> MKLAQGAFVDVIRIGALSPPTDQRSLWARTLLSEAVDQGLDSLPVPLQDVSTFTVTLQPALAVRLKALADQHNTPVSVYAAGLIEAMRRRSESGSVAEAPMELPADALPGEGAVREVLRPLLKQAAEKTAAGKIVFAEAATGTGKGRMIASLAAAAAIKGDTVVVSAPLAVTWQLVNDMKDIPEVRRVGLTLSLGRPNFISPQRTLEWAIDNERADLAAWIEGGGKPLSLRSMETSKVISHELCWLLEDALLLAEDLPADSLLLTSEDPADCPAQQLYVAMRSNYTEAGIILCSHFMLAAHTRMMQMRGLGNDEELDDEAPTGLSLPHFIDTLIVDEAHLLEQAFASVYTHT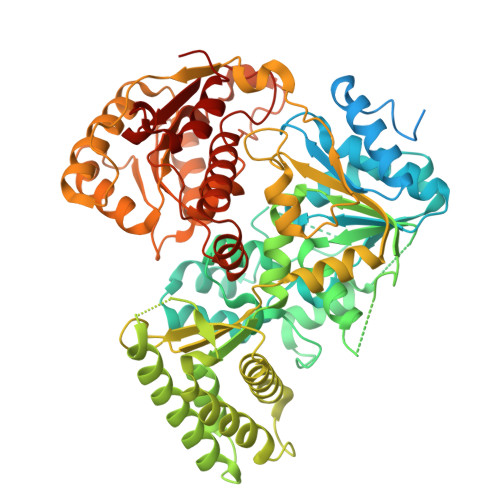LRLRPLMRTIEGLGSRGRKPALDALKELFTQMQVASARSTNTSLNVPLSDVPELIPALKDTVKTLGALPTKGMSRDARSVIRIATRAANDALSGHSRLRIEVTPVHSYPMLLSGRSNLQRALLGLWNATGGATLVSATLFTTGDNGSLTRWKLEVPTERAAFLPPVHPAWTTAPVLLHKEFCAHEPDDSPEWATECAQTIQGVASTAQGGTLVLCTSYQNTELLAGRLGAALGDRLIVQSKTSSAATCLAQFKAKHKAGIRPVWLGLGAAWTGIDLSDHSLPDNPELDRLLSDLVITRIPVGQNRSLTHERRTAIGGFRIISQEAAWHFRQGLGRLVRRPGVTHKNLWVLDARIYGGAAWVAPFRQILDRYKKA> GSMPPQLHNGLDFSAKVIQGSLDSLPQEVRKFVEGNAQLCQPEYIHICDGSEEEYGRLLAHMQEEGVIRKLKKYDNCWLALTDPRDVARIESKTVIITQEQRDTVPIPKSGQSQLGRWMSEEDFEKAFNARFPGCMKGRTMYVIP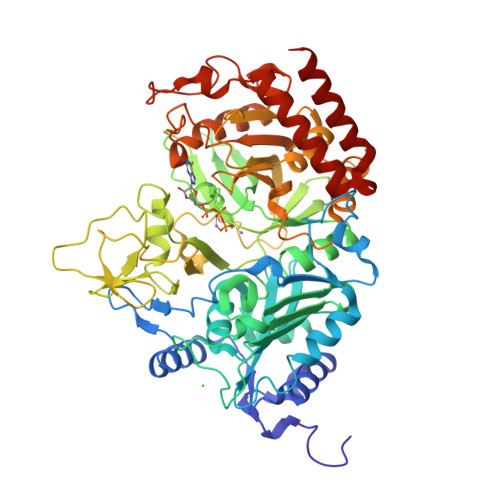FSMGPLGSPLAKIGIELTDSPYVVASMRIMTRMGTSVLEALGDGEFIKCLHSVGCPLPLKKPLVNNWACNPELTLIAHLPDRREIISFGSGYGGNSLLGKKCFALRIASRLAKEEGWLAEHMLILGITNPEGKKKYLAAAFPSACGKTNLAMMNPTLPGWKVECVGDDIAWMKFDAQGNLRAINPENGFFGVAPGTSVKTNPNAIKTIQKNTIFTNVAETSDGGVYWEGIDEPLAPGVTITSWKNKEWRPQDEEPCAHPNSRFCTPASQCPIIDPAWESPEGVPIEGIIFGGRRPAGVPLVYEALSWQHGVFVGAAMRSEATAAAEHKGKVIMHDPFAMRPFFGYNFGKYLAHWLSMAHRPAAKLPKIFHVNWFRKDKNGKFLWPGFGENSRVLEWMFGRIEGEDSAKLTPIGYVPKEDALNLKGLGDVNVEELFGISKEFWEKEVEEIDKYLEDQVNADLPYEIERELRALKQRISQM>[4x]MKRLETLESILERLRMSIKKNGLKNSKQ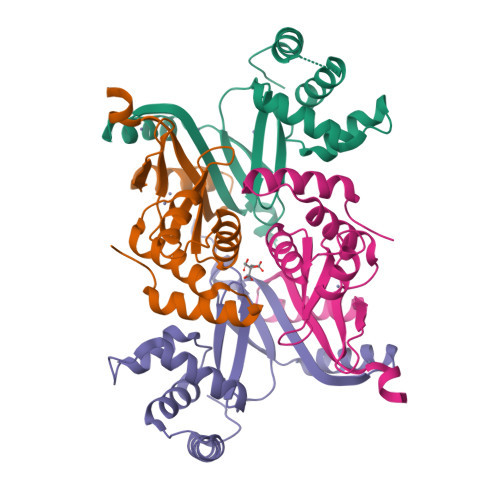REEVVSVLYRSGTHLSPEEITHSIRQKDKNTSISSVYRILNFLEKENFISVLETSKSGRRYEIAAKEHHDHIICLHCGKIIEFADPEIENRQNEVVKKYQAKLISHDMKMFVWCKECQESES In cochlea, deafness-related protein PDZD7 is an indispensable component of the ankle link complex, which is critical for the maturation of inner-ear hair cell for sound perception. FCHSD2 is expressed in hair cell and localizes along the stereocilia in a punctuate pattern, where it co-operates with CDC42 and N-WASP in regulating apical cell protrusion formation. At the extreme C-terminus of FCHSD2, there is a type I PDZ-binding motif (PBM, a.a. sequence Ile–Thr–Leu–Val) for associating with PDZ-containing protein. In this study, we uncover the interaction between FCHSD2 and PDZD7 through yeast two-hybrid screening and further verify the interaction using Coimmunoprecipitation (Co-IP) assays.

We proceed to solve the complex crystal structure of FCHSD2 tail/PDZD7 PDZ3 by the molecular replacement method at the resolution of 2.0 Å. Each asymmetric unit contains two complex molecules. Consistent with our biochemical characterization, the FCHSD2 tail/PDZD7 PDZ3 complex shows a 1 : 1 stoichiometry in the crystal structure. Five antiparallel β strands (βA–βE) form an open β-barrel, which is packed with two α-helices (αA and αB). FCHSD2 tail stretches along the groove in antiparallel with βB and inserts into the hydrophobic pocket of PDZD7 PDZ3. FCHSD2 tail forms the complex with PDZD7 PDZ3 that buries a total interface area of 526.6 Å2. Val740 from FCHSD2 tail inserts into the hydrophobic pocket of PDZD7 PDZ3 to form hydrophobic interactions with Leu868, Ile870, Ile872, and Val924 of PDZD7. The main chain atoms of Ile870, Ile872, and Gly874 from the βB form hydrogen bonds with Val740, Thr738, and Glu736 from FCHSD2, and stabilize the interaction. Intriguingly, in the FCHSD2/PDZD7 structure, Gly869 and Ile870 at the carboxylate-binding loop provide amide nitrogens to interact with the carbonyl oxygens of Val740 via a highly ordered water molecule. Arg928 also participates in interactions with the carboxylate to further stabilize the terminal carboxylate group.

>GPGSRIAEEAVGNVSTGALRTITLSKMKQSLGISISGGIESKVQPMVKIEKIFPGGAAFLCGDLQAGFELVAVDGESLEQVTHQRAVDTIRRAYRNKAREPMELVVRVP[2x];>[2x]GPGSTEKMEDVEITLV> MKHTELRAAVLDALEKHDTGATFFDGRPAVFDEADFPAVAV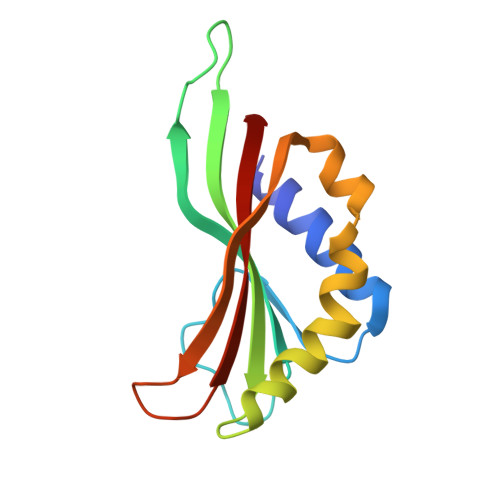YLTGAEYTGEELDSDTWQAELHIEVFLPAQVPDSELDAWMESRIYPVMSDIPALSDLITSMVASGYDYRRDDDAGLWSSADLTYVITYEM>[2x]DPYWAYSGAYGPEHWVTSSVSCGGSHQSPIDILDHHARVGDEYQELQLDGFDNESSNKTWMKNTGKTVAILLKDDYFVSGAGLPGRFKAEKVEFHWGHSNGSAGSEHSVNGRRFPVEMQIFFYNPDDFDSFQTAISENRIIGAMAIFFQVSPRDNSALDPIIHGLKGVVHHEKETFLDPFILRDLLPAS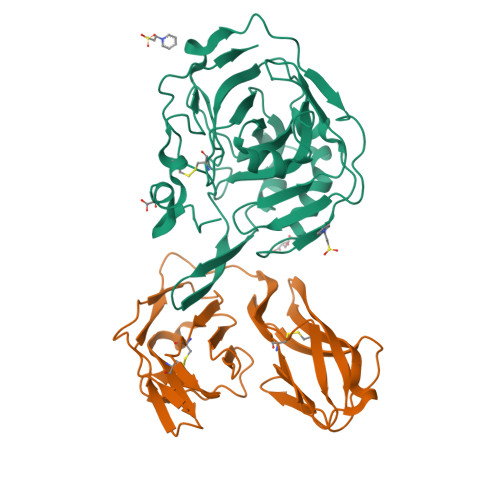LGSYYRYTGSLTTPPCSEIVEWIVFRRPVPISYHQLEAFYSIFTTEQQDHVKSVEYLRNNFRPQQALNDRVVSKS;>[2x]SAYIEDFETKTRSTVSVREGQGVVLLCGPPPHFGELSYAWTFNDSPLYVQEDKRRFVSQDTGNLYFAKVEPSDVGNYTCFVTNKEAHRSVQGPPTPLVLRTDGVMGEYEPKIEVRFPETIQAAKDSSIKLECFALGNPVPDISWKRLDGSPMPGKIKYSKSQAILEIPKFQQEDEGFYECIAGNLRGRNLAKGQLIFYA>[2x]GPTPEAPYASLTEIEHLVQSVCKSYRETCQLRLEDLLRQRSNIFSREEVTGYQRKSMWEMWERCAHHLTEAIQYVVEFAKRLSGFMELCQNDQIVLLKAGAMEVVLVRMCRAYNADNRTVFFEGKYGGMELFRALGCSELISSIFDFSHSLSALHFSEDEIALYTALVLINAHRPGLQEKRKVEQLQYNLELAFHHHLCKTHRQSILAKLPPKGKLRSLCSQHVERLQIFQHLHPIVVQAAFPPLYKELF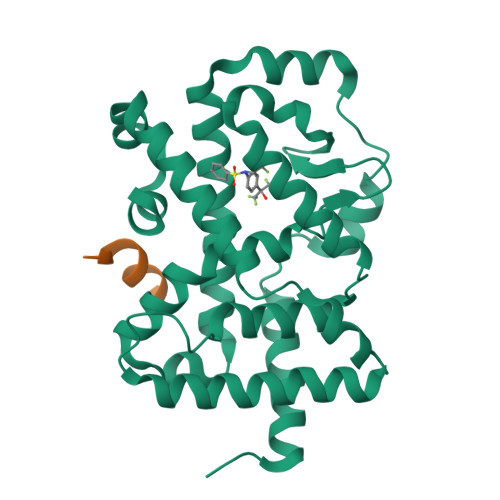STETESPVGLSK;>[2x]VESEFPYLLSLLGEVSPQP>[2x]MSQARPATVLGAMEMGRRMDVTSSSASVRAFLQRGHTEIDTAFVYANGQSETILGDLGLGLGRSGCKVKIATKAAPMFGKTLKPADVRFQLETSLKRLQCPRVDLFYLHFPDHGTPIEETLQACHQLHQEGKFVELGLSNYVSWEVAEICTLCKKNGWIMPTVYQGMYNAITRQVETELFPCLRHFGLRFYAF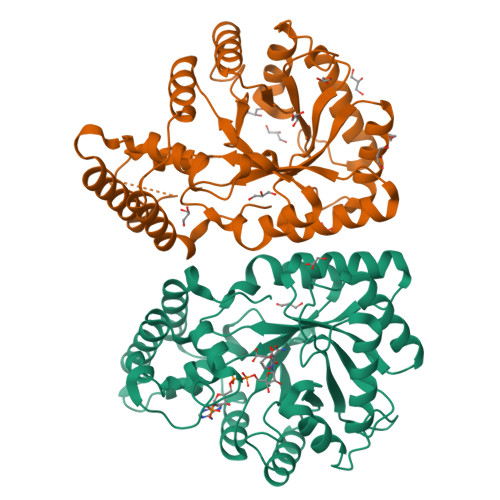NPLAGGLLTGRYKYQDKDGKNPESRFFGNPFSQLYMDRYWKEEHFNGIALVEKALKTTYGPTAPSMISAAVRWMYHHSQLKGTQGDAVILGMSSLEQLEQNLALVEEGPLEPAVVDAFDQAWNLVAHECPNYFR>GGQQMGRGSMTRRIRIGGAQMGAISRSDSKKEIVDRLIALLRQASEKGCELVVFPELALSTFFPRWYAERDGMDGYFEDGMPNAATLPLFEEARRLGIGFSLGYAELVQEDGRVRRFNTTVLVERNGEIVGKYRKIHLPGHAEYEPERSHQHLEKRYFEVGNTGFQVWDAFGGRVGMAICNDRRWVETYRVMGLQNVELILIGYNTPVNDSLSGEAETLGMFHNHLTMQAGAYQNSTWVVGVAKAGVEDGHRLMGGSVIVAPTGEIVAQAMTEGDELIVADCDLDRCRYYKSHIFNF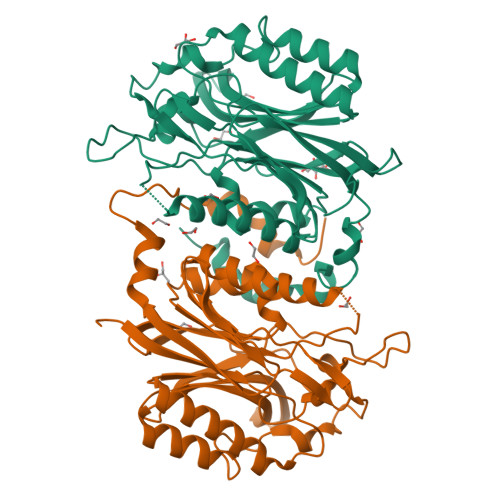AAHRRPEFYQRITSQTGVE[2x]>[2x]MNGDETKKVESEYIKKHHRHELVE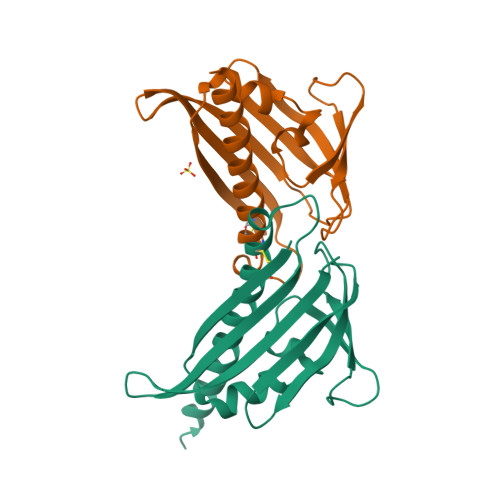SQCSSTLVKHIKAPLHLVWSIVRRFDEPQKYKPFISRCVVQGKKLEVGSVREVDLKSGLPATKSTEVLEILDDNEHILGIRIVGGDHRLKNYSSTISLHSETIDGKTGTLAIESFVVDVPEGNTKEETCFFVEALIQCNLNSLADVTERLQAESMEKKILEHHHHHH> MALTKAEMSEYLFDKLGLSKRDAKELVELFFEEIRRALENGEQVKLSGFGNFDLRDKNQRPGRNPKTGEDIPITARRVVTFRPGQKLKSRVENASPKDE;> MTKSELIERLATQQSHIPAKTVEDAVKEMLEHMASTLAQGERIEIRGFGSFSLHYRAPRTGRNPKTGDKVELEGKYVPHFKPGKELRDRANIYG;>MKRFGTRSATGKMVKLKLPVDVESLLIEASNRSGRSRSFEAVIRLKDHLHRYPKFNRAGNIYGKSLVKYLTMRLDDETNQLLIAAKNRSGWCKTDEAADRVIDHLIKFPDFYNSEIFREADKEEDITFNTL[3x];> MEFELGTMMSIAQVRSAGSAGNFYTDKDNYYVLGSMGERWAGRGAEQLGLQGSVDKDVFTRLLEGRLPDGADLSRMQDGSNRHRPGYDLTFSAPKSVSMMAMLGGDKRLIDAHNQAVDFAVRQVEALASTRVMTDGQSETVLTGNLVMALFNHDTSRDQEPQLHTHAVVANVTQHNGEWKTLSSDKVGKTGFIENVYANQIAFGRLYREKLKEQVEALGYETEVVGKHGMWEMPGVPVEAFSGRSQTIREAVGEDASLKSRDVAALDTRKSKQHVDPEIKMAEWMQTLKETGFDIRAYRDAADQRADLRTLTPGPASQDGPDVQQAVTQAIAGLSERKVQFTYTDVLARTVGILPPENGVIERARAGIDEAISREQLIPLDREKGLFTSGIHVLDELSVRALSRDIMKQNRVTVHPEKSVPRTAGYSDAVSVLAQDRPSLAIVSGQGGAAGQRERVAELVMMAREQGREVQIIAADRRSQMNMKQDERLSGELITGRRQLLEGMAFTPGSTVIVDQGEKLSLKETLTLLDGAARHNVQVLITDSGQRTGTGSALMAMKDAGVNTYRWQGGEQRPATIISEPDRNVRYARLAGDFAASVKAGEESVAQVSGVREQAILTQAIRSELKTQGVLGLPEVTMTALSPVWLDSRSRYLRDMYRPGMVMEQWNPETRSHDRYVIDRVTAQSHSLTLRDAQGETQVVRISSLDSSWSLFRPEKMPVADGERLRVTGKIPGLRVSGGDRLQVASVSEDAMTVVVPGRAEPATLPVSDSPFTALKLENGWVETPGHSVSDSATVFASVTQMAMDNATLNGLARSGRDVRLYSSLDETRTAEKLARHPSFTVVSEQIKTRAGETSLETAISHQKSALHTP

The nucleoprotein complex termed relaxosome contains the relaxase and other auxiliary transfer proteins, which assembles at the “origin of transfer” (oriT) region of a plasmid and prepares it for transfer to another bacterial cell. The F plasmid relaxosome complex contains, in addition to oriT, three plasmid-encoded proteins including the DNA-processing enzyme TraI (generally known as the “relaxase”) and 2 accessory proteins TraY and TraM, and IHF, a protein encoded by the bacterial genome. TraI is a multi-domain protein that consists of an N-terminal trans-esterase (TE) domain that contains its “relaxase” activity, followed by two helicase domains (one vestigial (VH), the other active (AH)), and a C-terminal domain (CTD) responsible for interactions with TraM. Here, we describe the cryo-EM structure of the fully assembled relaxosome encoded by the paradigm F plasmid in two different states corresponding to distinct functional steps along the DNA processing reaction.

Additional densities were observed in the “global” density map of the ss-27_+8ds+9_+143-R complex. These additional densities may correspond to the AH and CTD domains of TraI or/and to TraM, a protein that is also part of the complex. Near atomic resolution was not achieved for the AH and CTD domains, nonetheless we were able to locate these domains within the relaxosome. Apparently, this region makes no specific and stabilising contacts with proteins or DNA nearby.> MSQRITIDPVTRIEGHLRIDCEIENGVVSKAWASGTMWRGMEEIVKNRDPRDAWMIVQRICGVCTTTHAISSVRAAESALNIDVPVNAQYIRNIILAAHTTHDHIVHFYQLSALDWVDITSALKADPAKASAMLNGVSTWHLNSAEEFTKVQNKIKDLVASGQLGIFANGCWGHPAMQLPPEVNLIAVAHYLQALECQRDANRVVALLGGKTPHIQNLAVGGVANPINLDGLGVLNLERLMYIKSFIDKLSDFVEQVYKVDTAVIAAFYPEWLERGQGAVNYLSAPEFPTDGKNGSFLFPGGYITDADLSTYRPITSHSDEYLIKGIQESAKHAWYKDEAPQAPWEGTTVPDYTGWSDDGKYSWVKAPTFYGKTVEVGPLANMLCKLAAKRESTHAKLNEIVAIYTKLTGKTIEVAQLHSTLGRIIGRTVHCCELQNVLQDQYNALIVNIGKGDHTTFVKPDIPATGEFK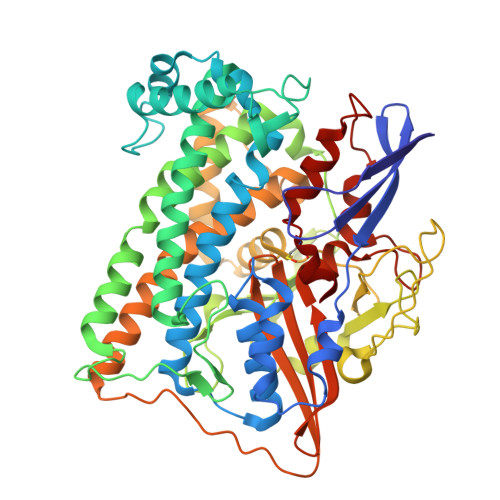GVGFLEAPRGMLSHWMVIKDGIISNYQAVVPSTWNSGPRNFNDEVGPYERSLVGTPIADPNKPLEVVRTIHSFDPCMSCAVH> MRRHYRDLIRNTPMPDTPQ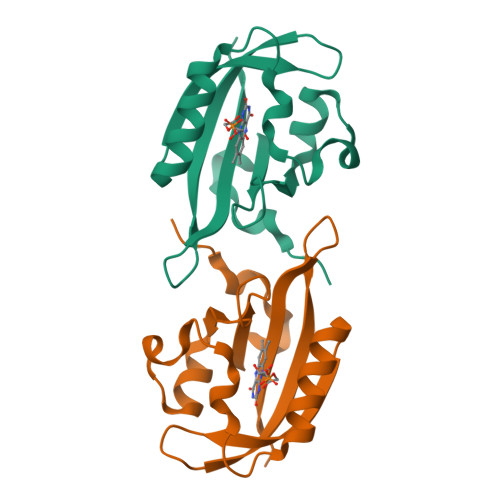DIADLRALLDEDEAEMSVVFSDPSQPDNPSIYVSDAFLVQTGYTLEEVLGRNCRFLQGPDTNPHAVEAIRQGLKAETRFTIDILNYRKDGSAFVNRLRIRPIYDPEGNLMFFAGAQNPVLEHHHHHH>[2x]PEFLNNTEPLCNVSGFAIVSKDNGIRIGSRGHVFVIREPFVACGPTECRTFFLTQGALLNDKHSNNTVKDRSPYRALMSVPLGSSPNAYQAKFESVAWSATACHDGKKWLAVGISGADDDAYAVIHYGGMPTDVVRSWRKQILRTQESSCVCMNGNCYWVMTDGPANSQASYKIFKSHEGMVTNEREVSFQGGHIEECSCYPNLGKVECVCRDNWNGMNRPILIFDEDLDYEVGYLCAGIPTD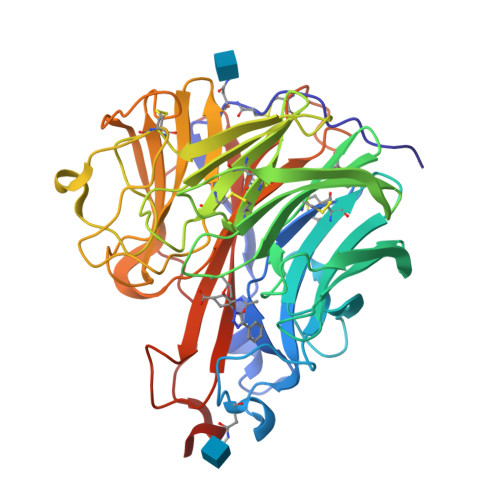TPRVQDSSFTGSCTNAVGGSGTNNYGVKGFGFRQGNSVWAGRTVSISSRSGFEILLIEDGWIRTSKTIVKKVEVLNNKNWSGYSGAFTIPITMTSKQCLVPCFWLEMIRGKPEERTSIWTSSSSTVFCGVSSEVPGWSWDDGAILPFDIDKM>[4x]MTVKYTDAQIQRLREYGNGTYEQKVFEDLASRDAAFSKEMSVASTDNEKKIKGMIANPSRHGLTQLMNDIADALVAEGFIEVRTPIFISKDALARMTITEDKPLFKQVFWIDEKRALRPMLAPNLYSVMRDLRDHTDGPVKIFEMGSCFRKESHSGMHLEEFTMLNLVDMGPRGDATEVLKNYISVVMKAAGLPDYDLVQEESDVYKETIDVEINGQEVCSAAVGPHYLDAAHDVHEPWSG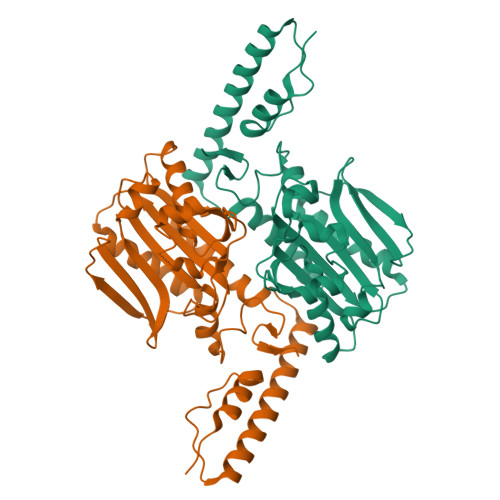AGFGLERLLTIREKYSTVKKGGASISYLNGAKINGSHHHHHH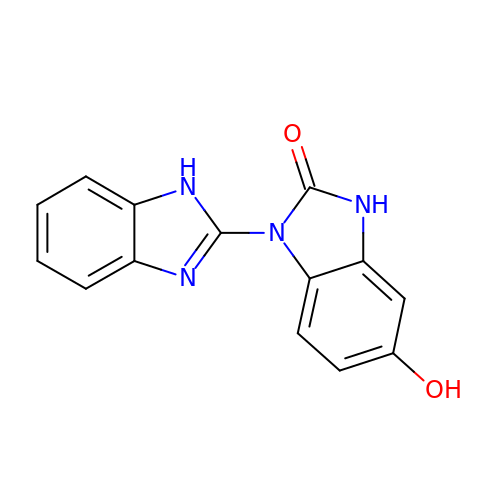5-hydroxy-1'H-1,2'-bibenzimidazol-2(3H)-one | C14 H10 N4 O2 | YOEAQWYCBDUGQE-UHFFFAOYSA-N>[4x]GHFKDPKRLYCKNGGFFLR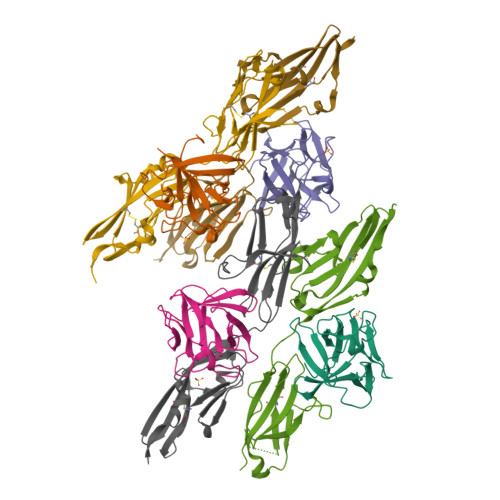IHPDGRVDGVREKSDPHIKLQLQAEERGVVSIKGVSANRYLAMKEDGRLLASKSVTDECFFFERLESNNYNTYRSRKYTSWYVALKRTGQYKLGSKTGPGQKAILFLPMSAKS;>NSNNKRAPYWTNTEKMEKRLHAVPAANTVKFRCPAGGNPMPTMRWLKNGKEFKQEHRIGGYKVRNQHWSLIMESVVPSDKGNYTCVVENEYGSINHTYHLDVVERSPHRPILQAGLPANASTVVGGDVEFVCKVYSDAQPHIQWIKHVEKNGSKYGPDGLPYLKVLKAAGVNTTDKEIEVLYIRNVTFEDAGEYTCLAGNSIGISFHSAWLTVLPAPGRE[4x]>GPLGSNNVNDLITVTKQMITEGIKDDGVIQAHDGEHIIYTSDFKIDNAVKAGDTMTVKYDKHTIPSDITDDFTPVDITDPSGEVIAKGTFDLNTKTITYKFTDYVDRYENVNAKLELNSYIDKKEVPNETNLNLTFATADKETSKNVKVEYQKPIVKDESNIQSIFSHLDTTKHEVEQTIYVNPLKLNAKNTNVTIKSGGVADNGDYYTGDGSTIIDSNTEIKVYKVASGQQLPQSNKIYDYSQYEDVTNSVTINKNYGTNMANINFGDIDSAYIVKV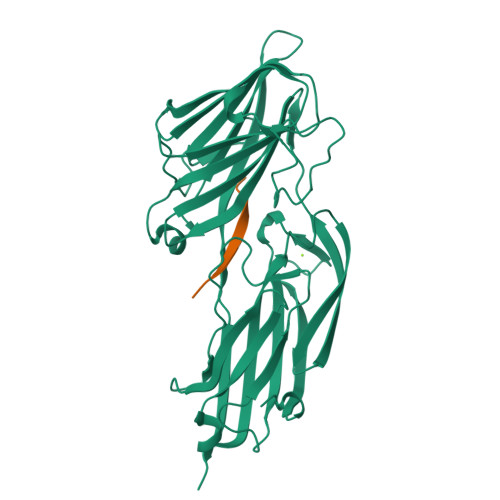VSKYTPGAEDDLAVQQGVRMTTTNKYNYSSYAGYTNTILSTTDSGGGDGTVKP[2x];>SKQFTSSTSYNRGDS[2x]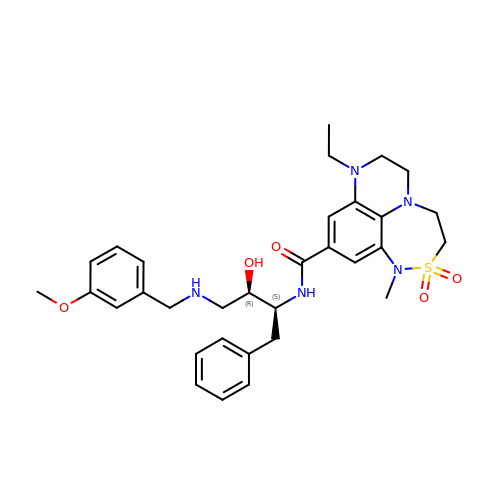N-{(1S,2R)-1-BENZYL-2-HYDROXY-3-[(3-METHOXYBENZYL)AMINO]PROPYL}-8-ETHYL-1-METHYL-3,4,7,8-TETRAHYDRO-1H,6H-[1,2,5]THIADIAZEPINO[5,4,3-DE]QUINOXALINE-10-CARBOXAMIDE 2,2-DIOXIDE | C32 H41 N5 O5 S | UKAHVQYVCSVAKY-BHBYDHKZSA-N> DERADTQRQLEQTQKDIGELKKLLDGIQQEKSGVQKQLKSTETEMGDLEKQIKALQDELDKSEAELKRLDGEKKKLQDARIEQQRLLAIQARAAYQSGREEYLKLLLNQEHPEKFSRTLTYYDYINKARLEQLASFNETLRQLANVEQDISAQKAEQLSKQGELDSRREALAATRKERQQALAKLNSDYRERDQKLKSRQQDQAELAKVLRTIEETLARQAREAAAAAERERQRALAAERERARQQQAAPGRVTSPPREPAPGPLVSSTGAVYGGAFG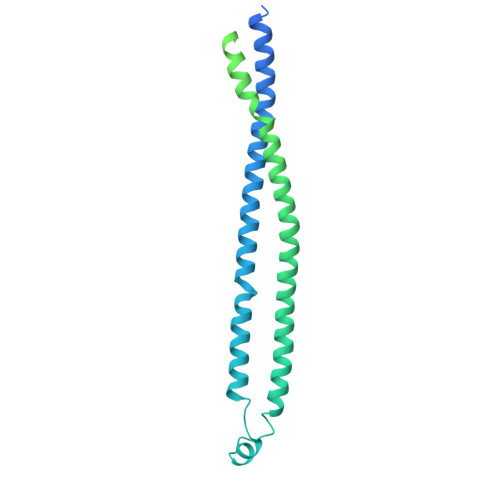SARGKLPWPVNGRVVARFGSQRGDDPRAKWDGVLISASAGSTVRAVHGGRVVFADWLRGAGLLVILDHGGGYLSLYGHNQSLLKDAGDTVKAGDPIATVGTSGGQSSPAVYFAIRHQGRPADPTTWCRAQG> MHRRVKVLLYGQVV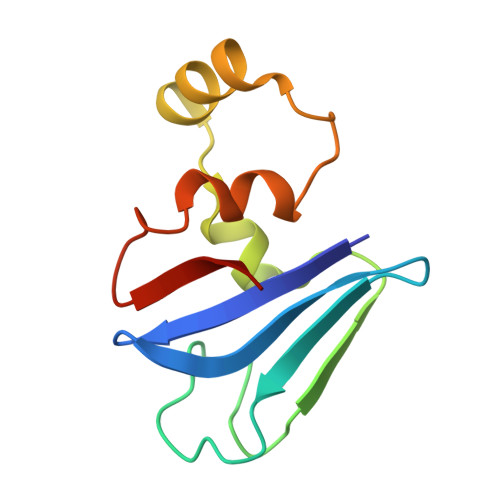GELSQNDSGFLFQYAHDYHGPAISISLPVAQRQFPSETLHPYFASLAPEGWLRQRYSQIQHRDENDLLGMLIDNGKNLLGAIQILPWEE>MAGPLSGLRVVELAGIGPGPHAAMILGDLGADVVRIDRPSSVDGISRDAMLRNRRIVTADLKSDQGLELALKLIAKADVLIEGYRPGVTERLGLGPEECAKVNDRLIYARMTGWGQTGPRSQQAGHDINYISLNGILHAIGRGDERPVPPLNLVGDFGGGSMFLLVGILAALWERQSSGKGQVVDAAMVDGSSVLIQMMWAMRATGMWTDTRGANMLDGGAPYYDTYECADGRYVAVGAIEPQFYAAMLAGLGLDAAELPPQNDRARWPELRALLTEAFASHDRDHWGAVFANSDACVTPVLAFGEVHNEPHIIERNTFYEANGGWQPMPAPRFSRTASSQPRPPAATIDIEAVLTD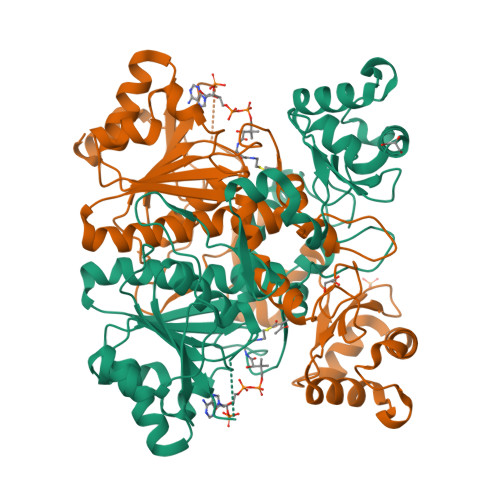WDG[4x]> MQNKTTASKSWVGTWATAPQLVEPRNMPPAPGLTNSTLRQVVCVSIGGKQLQFRFSNRFSKSPVTMKTVHIAVSKGGSEIEPSTSKELTFNGQPDVTMEPGKAVISDPISFNLKPRMLVAITISFGETSPDVTGHPGSRTTSYLLAGDQSSPDADFSQAVKTDHWYVINGIDLMAQKRAAAIAILGNSITDGRGSGTNKQDRWPDELALRLLKNKRTRDIGVLNMGIGGNCVLHGGLGPTALSRFNRDILKQHGVRWLIIFEGVNDIGGTPDKEAADKVAQGLIAAYDKMIDEAHAKGIKVYGGTITPIKKSFYYKDYRETARQTVNKWIRTSGHFDAVIDFDKAMRNPKDTLT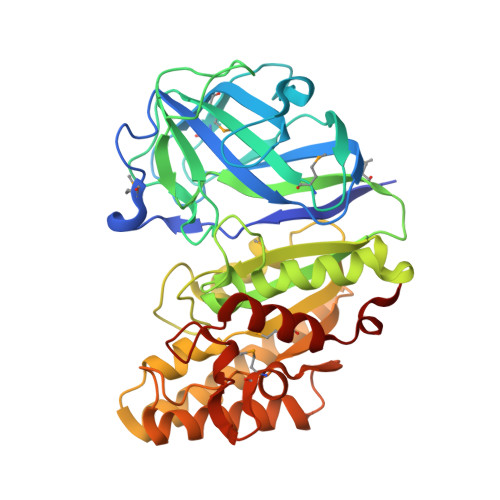LRPEAQSGDYLHPNELGYRIMAGAIDLSLFKE>NEAIECHLSDLLQQLTSVNASKPSERGLVRQEEAEDPACIPIFWVSKWVDYSDKYGLGYQLCDNSVGVLFNDSTRLILYNDGDSLQYIERDGTESYLTVSSHPNSLMKKITLLNYFRNYMSEHLLKAGANITPREGDELARLPYLRTWFRTRSAIILHLSNGTVQINFFQDHTKLILCPLMAAVTYINEKRDFQTYRLSLLEEYGCCKELASRLRYARTMVDKLLSSRSASNRLKAS[2x];>[2x]FSQHKTSTI

One of CSFs, Emi2 (also known as F-box only protein 43) inhibits APC/C activity by binding to APC/C-cdc20; therefore, Emi2 blocks the ubiquitin-mediated proteolysis of MPF8910. Subsequently, the phosphorylated threonines in Emi2 can be recognized by Plk1, which undergoes phosphorylation, and these phosphorylated sites serve as a recognition site for SCF, another class of ubiquitin ligases; SCF destabilizes Emi2 and activates APC/C10. In this study, one of our aim was to elucidate recognition of Emi2 by the Polo-box domain (PBD) of Plk1 using X-ray crystallography and biochemical characterization. To elucidate the detailed molecular mechanism of recognition of Emi2 by Plk1-PBD, we determined structure of the complexes of PBD domain (367–603 of Plk1) with peptides Emi2146–177 or Emi2169–177.

Because we could not identify the binding mode of phospho-Thr176 in the structure of the complex of PBD with Emi2146–177, we crystallized a shorter phosphopeptide (Emi2169–177, containing a single phospho-Thr176) with PBD and solved the crystal structure of this complex at 1.8 Å. In the asymmetric unit of the crystal structure, two molecules of Plk1-PBD bound with the one Emi2 peptide, respectively were found molecule 1 (shown in blue in Fig. 2D) displayed the whole sequence of amino acids (169 to 177) corresponding to Emi2169–177, while molecule 2 appeared as 172HKTSpTI177 of Emi2. After careful analysis of the structure of this complex (Right), it is clear that the phosphothreonine residue (Thr176) binds to the canonical phospho-Thr/Ser-binding pocket of PBD; this mechanism is very similar to the known structures of binding complexes like PBIP1·PBD25 or cdc25C·PBD24. Phe169 was found to be located in hydrophobic pockets, which are characterized by the presence of three tyrosine residues (Tyr417, Tyr481, and Tyr485). This binding behavior is different from that of peptides from native proteins including cdc25C·PBD24 or PBIP1·PBD25. As far as we know, ours is the first report of natural peptides occupying these hydrophobic pockets in Plk1-PBD. To elucidate characteristics of the possible protein-protein interaction site in Plk1-PBD, we mapped sequence conservation scores calculated from the multiple-sequence alignment of various Plk1 homologs onto the surface of Plk1. The two interacting binding pockets, such as the phospho-binding pocket and tyrosine-rich hydrophobic pockets, are located in the middle of an evolutionarily conserved region as shown in the structure of the complex in Fig. 2D. Especially, fluorescence decay of Phe169Ala mutant is minimal compared with two other mutants and wild type Emi2-mCherry, indicating that Phe169 in Emi2 is important for degradation of Emi2 after pathernogenetic activation. For example, Phe169 of Emi2 is located in the middle of a Tyr-rich hydrophobic pocket; this seems to be the first report that a natural peptide binds to Tyr-rich hydrophobic pocket.> MNNDNPLFKSAMVALSLKISIGNVVKTMQFEPSTMVYDACRMIRERIPEALAGPPNDFGLFLSDDDPKKGIWLEAGKALDYYMLRNGDTMEYRKKQRPLKIRMLDGTVKTIMVDDSKTVTDMLMTICARIGITNHDEYSLVRELMEEKKDELNWLDHGRTLREQGVEEHETLLLRRKFFYSDQNVDSRDPVQLNLLYVQARDDILNGSHPVSFDKACEFAGFQCQIQFGPHNEQ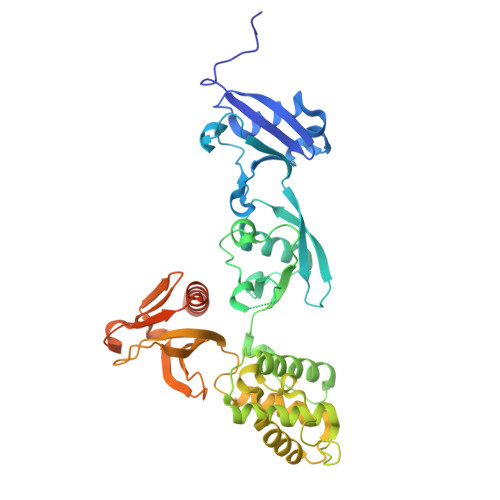KHKAGFLDLKDFLPKEYVKQKGERKIFQAHKNCGQMSEIEAKVRYVKLARSLKTYGVSFFLVKEKMKGKNKLVPRLLGITKECVMRVDEKTKEVIQEWSLTNIKRWAASPKSFTLDFGDYQDGYYSVQTTEGEQIAQLIAGYIRIILKKKKSKDHFGLEGDEESTMLEDSVSPKKST> MGSDAFDEMDEIWALYADDGAQALDAMEASLLALQAGEDAAAHVGPLFRAVHTFKGNSRVLGLSVVESRAHLCEDLIGLVRDAGVPMDGEIVEILLFASDTLRAMLEETAASRADVEG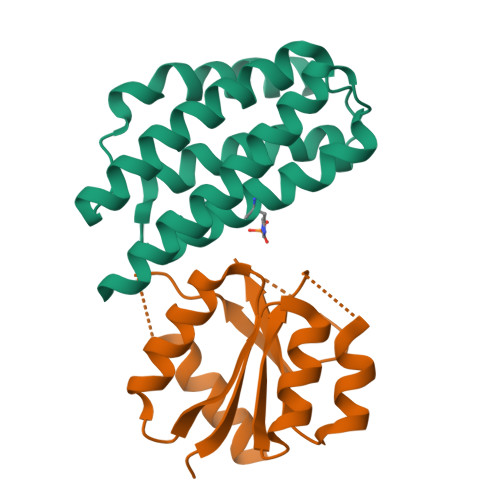TGSEALMDQLRSKIARCSRSHHHHHH;> MRGSHHHHHHGSPYNVMIVDDAAMMRLYIASFIKTLPDFKVVAQAANGQEALDKLAAQPNVDLILLNIEMPVMDGMEFLRHAKLKTRAKICMLASVAVSGSPHAARARELGADGVVAKPSGTVSHDLEEKTGGELARTMRTLMAA Ktr4p is a member of the Kre2/Mnt1 family of glycosyltransferases. Ktr4p, as the other members of the Kre2/Mnt1 family, is a type II membrane protein with a short N-terminal cytosolic tail and a large lumenal catalytic domain of 40 kDa, which is separated from the membrane by a stalk domain of 11 kDa. Ktr4p, with its large central β-sheet, belongs to the GT-A fold class of glycosyltransferases. We used GDP-mannose as the sugar donor, and tested mannose, α-1,2-mannobiose and methyl-α-mannoside as potential acceptors; in the case of both donor and acceptor this was based on suggestions from sequence identity. Our results, shown in Fig 4, confirm that Ktr4p is an active mannosyltransferase enzyme.

X-ray diffraction data for the apo structure was collected to 2.2 Å resolution and indexed in the space group P212121 with the unit cell dimensions a = 60.2 Å, b = 102.4 Å, c = 156.9 Å, α = β = γ = 90°. The Matthews' coefficient suggested the presence of two molecules per asymmetric unit (corresponding to a solvent content of 51%). The apo structure of Ktr4p contains no metals in the active site, but density corresponding to three metal ions was observed on the surface of monomer B. These metal ions, modelled as calcium in the deposited structure are grouped close together and are coordinated by the sidechains of Asp-77 and Asp-81, Asp-308 and Glu-311, and His-84 and Glu-311, respectively. They are involved in the formation of crystal contacts and are not near the active site; it is therefore likely that they are merely a result of crystal packing. In our structure, although the extreme N-terminus is not visible, part of the stalk domain, corresponding to helices α1 and α2, is clearly defined in the electron density. These helices protrude from the N-terminal subdomain of the protein and fold over the surface of the C-terminal subdomain, which has the effect of making the protein appear more like a large single domain structure. Three disulfide bonds are present in the C-terminal subdomain of the protein, between residues Cys-269 – Cys-427, Cys-345 – Cys-447 and Cys-417 – Cys-431; these likely provide significant additional stability to the subdomain. The complex structure shows that only slight changes occur in the Ktr4p structure upon ligand binding; the monomer structures of Ktr4p in the presence and absence of GDP and Mn2+ can be superimposed with a maximum RMSD of 0.37 Å over 386 Cα atoms (chain B of the apo structure superimposed on chain A of the complex structure).

>SMNENYLQAVKDSAKSQYASLRESYKSITGKTESADELPDHDAEVLDSIMDRLHEPLYEKDTFDPNEVLAENKQLYEEFLLQEISEPKVDNLVRSGDPLAGKAKGTILSLVRNSDLEDIISSIQQLEEEYNKNFGYPYTFLNDEEFTDEFKDGIKSILPKDRVVEFGTIGPDNWNMPDSIDRERYDQEMDKMSKENIQYAEVESYHNMCRFYSKEFYHHPLLSKYKYVWRLEPNVNFYCKINYDVFQFMNKNDKIYGFVLNLYDSPQTIETLWTSTMDFVEEHPNYLNVNGAFAWLKDNSQNPKNYDYTQGYSTCHFWTNFEIVDLDFLRSEPYEKYMQYLEEKGGFYYERWGDAPVRSLALALFADKSSIHWFRDIGYHHTPYTNCPTCPADSDRCNGNCVPGKFTPWSDLDNQNCQATWIRHSMSEEELEMY[2x]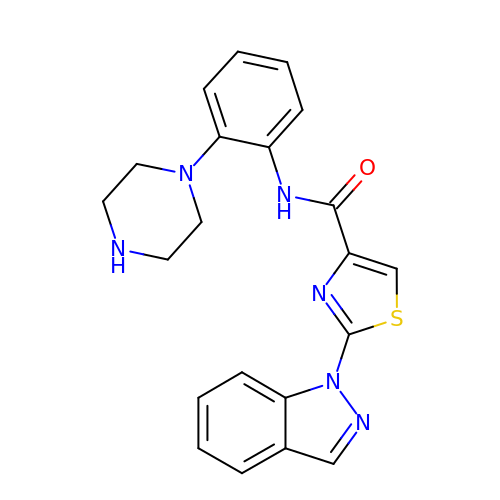2-(1H-indazol-1-yl)-N-[2-(piperazin-1-yl)phenyl]-1,3-thiazole-4-carboxamide | C21 H20 N6 O S | WQIZBWOPEUALCL-UHFFFAOYSA-N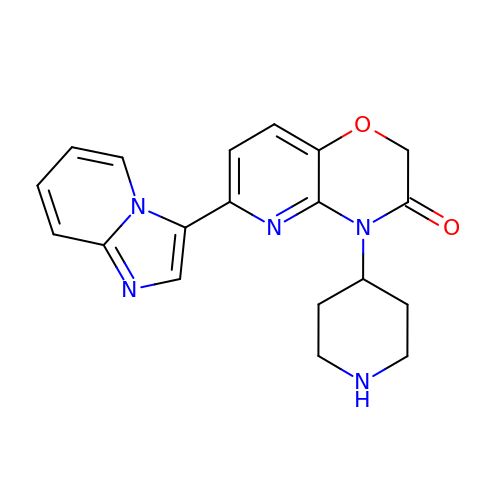(6P)-6-[(4R)-imidazo[1,2-a]pyridin-3-yl]-4-(piperidin-4-yl)-2H-pyrido[3,2-b][1,4]oxazin-3(4H)-one | C19 H19 N5 O2 | SQOLXUGRJNPDOA-UHFFFAOYSA-N>HMKHSDEYKIRRERNNIAARKSRDKAKMRNLETQHKVLELTAENERLQKKVEQLSRELSTLRNLFKQ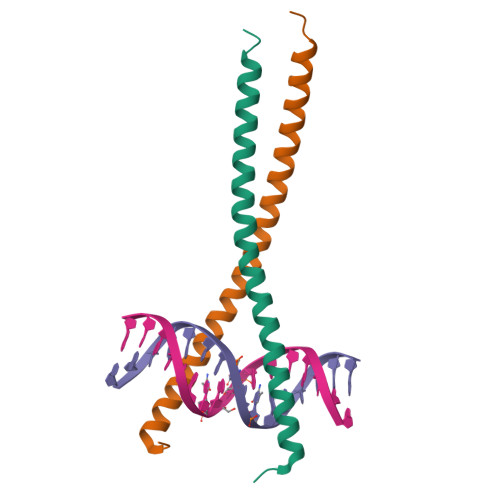LPEPLLASSGH[2x]> MKMTSIQQRAELHRQIWQIANDVRGSVDGWDFKQYVLGALFYRFISENFSSYIEAGDDSICYAKLDDSVITDDIKDDAIKTKGYFIYPSQLFCNVAAKANTNDRLNADLNSIFVAIESSAYGYPSEADIKGLFADFDTTSNRLGNTVKDKNARLAAVLKGVEGLKLGDFNEHQIDLFGDAYEFLISNYAANAGKSGGEFFTPQHVSKLIAQLAMHGQTHVNKIYDPAAGSGSLLLQAKKQFDNHIIEEGFFGQEINHTTYNLARMNMFLHNINYDKFDIKLGNTLTEPHFRD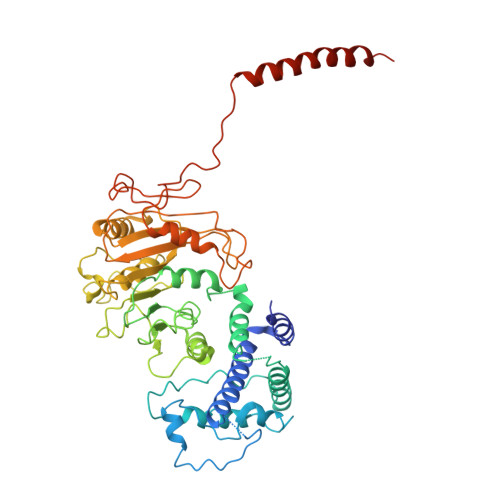EKPFDAIVSNPPYSVKWIGSDDPTLINDERFAPAGVLAPKSKADFAFVLHALNYLSAKGRAAIVCFPGIFYRGGAEQKIRQYLVDNNYVETVISLAPNLFFGTTIAVNILVLSKHKTDTNVQFIDASELFKKETNNNILTDAHIEQIMQVFASKEDVAHLAKSVAFETVVANDYNLSVSSYVEAKDNREIIDIAELNAELKTTVSKIDQLRKDIDAIVAEIEGCEVQK> KASEGLARVAALAR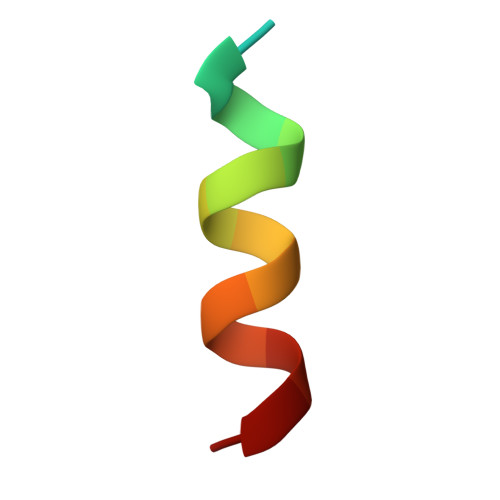SR> MTSRKKVLLKVIILGDSGVGKTSLMNQYVNKKFSNQYKATIGADFLTKEVMVDDRLVTMQIWDTAGLERFQSLGVAFYRGADCCVLVFDVTAPNTFKTLDSWRDEFLIQASPRDPENFPFVVLGNKIDLENRQVATKRAQAWCYSK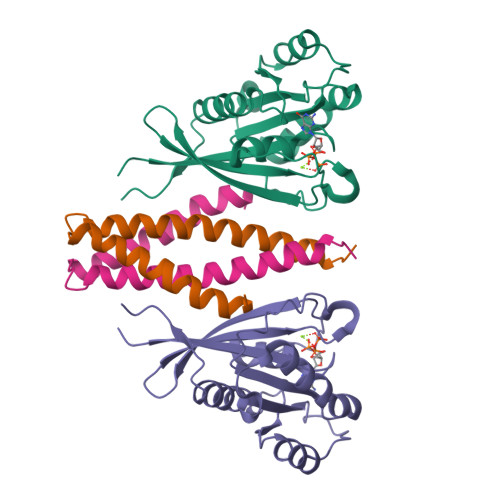NNIPYFETSAKEAINVEQAFQTIARNALKQETEVELYNEFPEPIKLDKNDRAKASAESCSC;> SREEFEQILQERNELKAKVFLLKEELAYFQRELLTDHRVPSLLLEAMKVAVRKQRKKIKAKMLGT> VTYEEEAVPAPVRGRLEVLSDLLYVASPDRAMVFTRTKAETEEIAQGLLRLGHPAQALHGDMSQGERERVMGAFRQGEVRVLVATD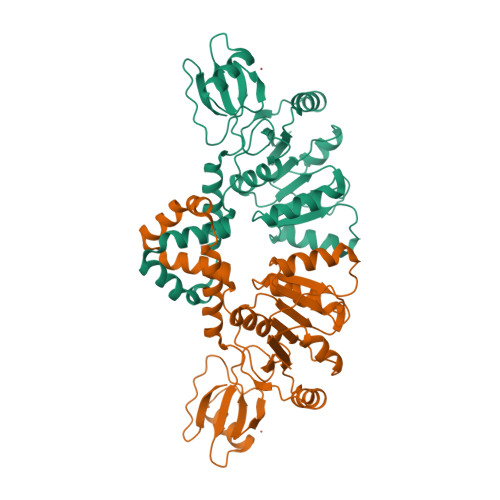VAARGLDIPQVDLVVHYRMPDRAEAYQHRSGRTGRAGRGGRVVLLYGPRERRDVEALERAVGRRFKRVNPPTPEEVLEAKWRHLLARLARVPEKDYRLYQDFAGRLFAEGRVEVVAALLALLLGGAPAERSLLTGEEGWRTYKATGPRLSLPRLVALLKGQGLEVGKVAEAEGGFYVDLRPEARPEVAGLRLEPARRVEGLLEIPSRTRRPARA> GSSHHHHHHMGNVFDYEDIQLIPAKCIVNSRSECDTTVTLGKHKFKLPVVPANMQTIIDERIATYLAENNYFYIMHRFQPEKRISFIRDMQSRGLIASISVGVKE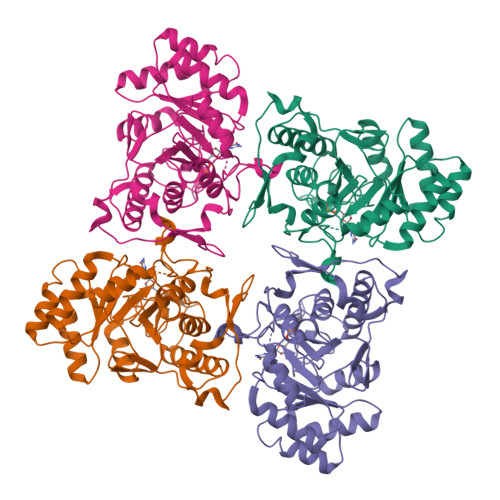DEYEFVQQLAAEHLTPEYITIDIAHGHSNAVINMIQHIKKHLPESFVIAGNVGTPEAVRELENAGADATKVGIGPGKVCITKIKTGFGTGGWQLAALRWCAKAASKPIIADGGIRTNGDVAKSIRFGATMVMIGSLFAGHEESPGETIEKDGKLYKEYFGSASEFQKGEKKNVEGKKMFVEHKGSLEDTLIEMEQDLQSSISYAGGTKLDSIRTVDYVVVKNSIFNGDKVY>MKLPVREFDAVVIGAGGAGMRAALQISQSGQTCALLSKVFPTRSHTVSAQGGITVALGNTHEDNWEWHMYDTVKGSDYIGDQDAIEYMCKTGPEAILELEHMGLPFSRLDDGRIYQRPFGGQSKNFGGEQAARTAAAADRTGHALLHTLYQQNLKNHTTIFSEWYALDLVKNQDGAVVGCTALCIETGEVVYFKARATVLATGGAGRIYQSTTNAHINTGDGVGMAIRAGVPVQDMEMWQFHPTGIAGAGVLVTEGCRGEGGYLLNKHGERFMERYAPNAKDLAGRDVVARSIMIEIREGRGCDGPWGPHAKLKLDHLGKEVLESRLPGILELSRTFAHVDPVKEPIPVIPTCHYMMGGIPTKVTGQALTVNEKGEDVVVPGLFAVGEIACVSVHGANRLGGNSLLDLVVFGRAAGLHLQESIAEQGALRDASESDVEASLDRLNRWNNNRNGEDPVAIRKALQECMQHNFSVFREGDAMAKGLEQLKVIRERLKNARLDDTSSEFNTQRVECLELDNLMETAYATAVSANFRTESRGAHSRFDFPDRDDENWLCHSLYLPESESMTRRSVNMEPKLRPAFPPKIRTY[3x];>[3x]MRLEFSIYRYNPDVDDAPRMQDYTLEADEGRDMMLLDALIQLKEKDPSLSFRRSCREGVCGSDGLNMNGKNGLACITPISALNQPGKKIVIRPLPGLPVIRDLVVDMGQFYAQYEKIKPYLLNNGQNPPAREHLQMPEQREKLDGLYECILCACCSTSCPSFWWNPDKFIGPAGLLAAYRFLIDSRDTETDSRLDGLSDAFSVFRCHSIMNCVSVCPKGLNPTRAIGHIKSMLLQRNA;>MIRNVKKQRPVNLDLQTIRFPITAIASIL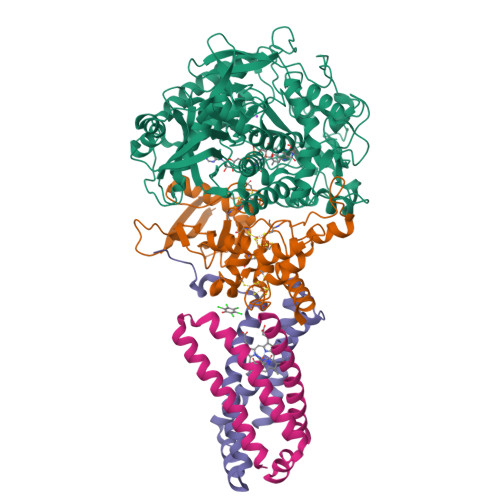HRVSGVITFVAVGILLWLLGTSLSSPEGFEQASAIMGSFFVKFIMWGILTALAYHVVVGIRHMMMDFGYLEETFEAGKRSAKISFVITVVLSLLAGVLVW[3x];>[3x]MVSNASALGRNGVHDFILVRATAIVLTLYIIYMVGFFATSGELTYEVWIGFFASAFTKVFTLLALFSILIHAWIGMWQVLTDYVKPLALRLMLQLVIVVALVVYVIYGFVVVWGV> GYQALEKYSRDLTALARAGKLDPVIGRDTEIRRAIQILSRRTKNNPILLGDPGVGKTAIVEGLAI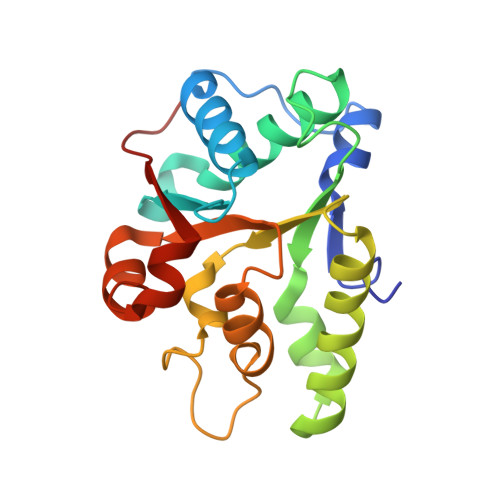KIVQGDVPDSLKGRKLVSLDLSSLIAGAKYRGDFEERLKSILKEVQDAEGQVVMFIDEIHTVVGAGAVAEGALDAGNILKPMLARGELRCIGATTVSEYRQFIEKDKALERRFQQILVEQPS> MSKKQPKPVKAEQLKSYYEESRGLERDLIGEFVKSRKTAWRVATASGLFGLLGMVCGIVGFSQPAPAPLVLRVDNATGAVDVVTTLREHESSYGEVVDTYWLNQYVLNREAYDYNTIQMNYDTTALLSAPAVQQDYYKLFDGSNARDRVLGNKARITVRVRSIQPNGRGQATVRFTTQQHNSNGTVEAPQHQIATIGYTYIGAPMRS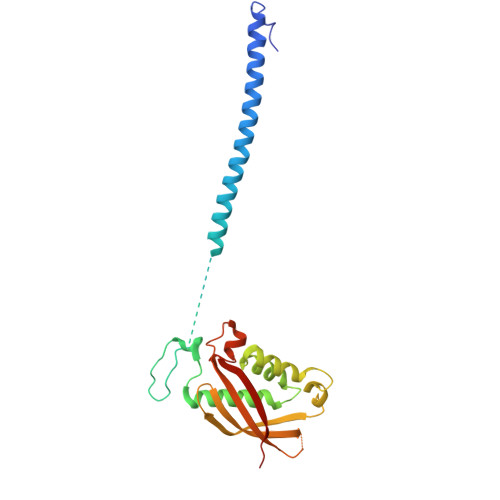SDRLLNPLGFQVTSYRADPEILNN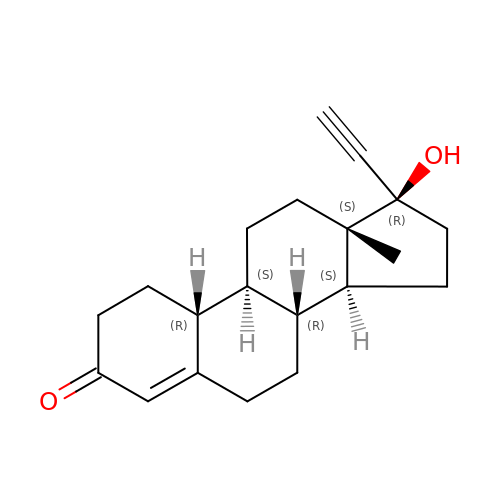(14beta,17alpha)-17-ethynyl-17-hydroxyestr-4-en-3-one | C20 H26 O2 | VIKNJXKGJWUCNN-XGXHKTLJSA-N> GVKTFQFPFAEQLEKVAEQFPTFQILNEEGEVVNEEAMPELSDEQLKELMRRMVYTRILDQRSISLNRQGRLGFYAPTAGQEASQIASHFALEKEDFILPGYRD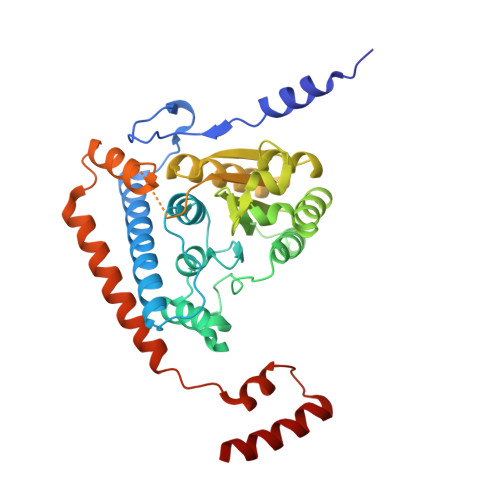VPQIIWHGLPLYQAFLFSRGHFHGNQIPEGVNVLPPQIIIGAQYIQAAGVALGLKMRGKKAVAITYTGDGGTSQGNFYQGINFAGAFKAPAIFVVQNNRFAISTPVEKQTVAKTLAQKAVAAGIPGIQVDGMDPLAVYAAVKAARERAINGEGPTLIETLCFRYGPHTMSGDDPTRYRSKELENEWAKKDPLVRFRKFLEAKGLWSEEEENNVIEQAKEEIKEAIKKADETPKQKVTDLISIMFEELPFNLKEQYEIYKEKESK> CTSIVAQDSRGHVYHGRNLDYPYGSILRKLTVDVQFLKNGQIAFTGTTFIGYVGLWTGQSPHKFTVSGDERDRGWWWENLVAALFLRHSPISWLLRTTLSEAESFEAAVYRLAKTPLIADVYYIVGGTNPREGVVITRNRDGPADIWPLDPLKGVWFLVETNYDHWKPAPEEDDRRTPAIKALNATGQAKLSLETLF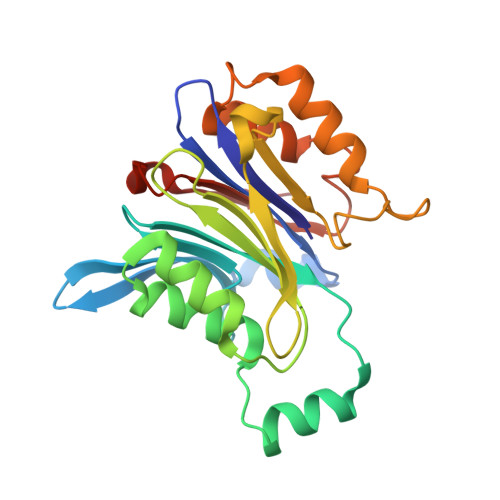QVLSVVPVYNNYTIYTTVMSAASPDKYMTRIRNPS>MPAPHGGILQDLIARDALKKNELLSEAQSSDILVWNLTPRQLCDIELILNGGFSPLTGFLNENDYSSVVTDSRLADGTLWTIPITLDVDEAFANQIKPDTRIALFQDDEIPIAILTVQDVYKPNKTIEAERVFRGDPEHPAISYLFNVAGDYYVGGSLEAIQLPQHYDYPGLRKTPAQLRLEFQSRQWDRVVAFQTRNPMHRAHRELTVRAAREANAKVLIH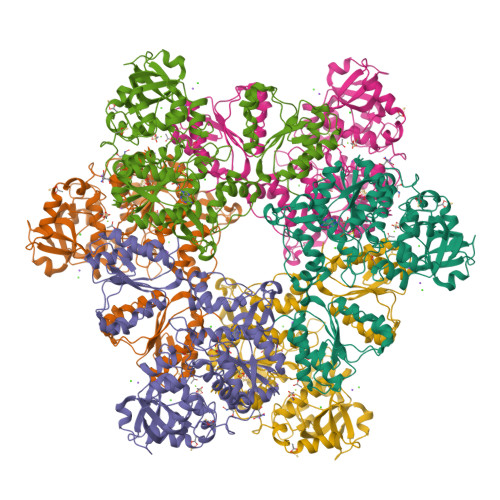PVVGLTKPGDIDHHTRVRVYQEIIKRYPNGIAFLSLLPLAMRMSGDREAVWHAIIRKNYGASHFIVGRDHAGPGKNSKGVDFYGPYDAQELVESYKHELDIEVVPFRMVTYLPDEDRYAPIDQIDTTKTRTLNISGTELRRRLRVGGEIPEWFSYPEVVKILRESNPPRPKQGFSIVLGNSLTVSREQLSIALLSTFLQFGGGRYYKIFEHNNKTELLSLIQDFIGSGSGLIIPDQWEDDKDSVVGKQNVYLLDTSSSADIQLESADEPISHIVQKVVLFLEDNGFFVF[2x]>MEIFKYMEKYDYEQLVFCQDEASGLKAVIAIHDTTLGPALGGARMWTYNAEEEAIEDALRLARGMTYKNAAAGLNLGGGKTVIIGDPFADKNEDMFRALGRFIQGLNGRYITAEDVGTTVDDMDLIHQETDYVTGISPAFGSSGNPSPVTAYGVYRGMKAAAKEAFGSDS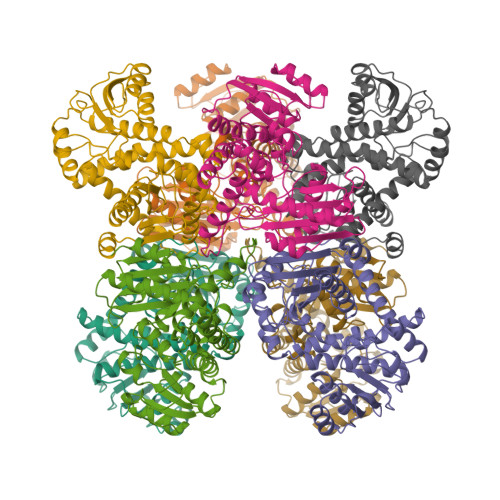LEGLAVSVQGLGNVAKALCKKLNTEGAKLVVTDVNKAAVSAAVAEEGADAVAPNAIYGVTCDIFAPCALGAVLNDFTIPQLKAKVIAGSADNQLKDPRHGKYLHELGIVYAPDYVINAGGVINVADELYGYNRTRAMKRVDGIYDSIEKIFAISKRDGVPSYVAADRMAEERIAKVAKARSQFLQDQRNILNGR[2x]> GSHMGNRTFSYTLED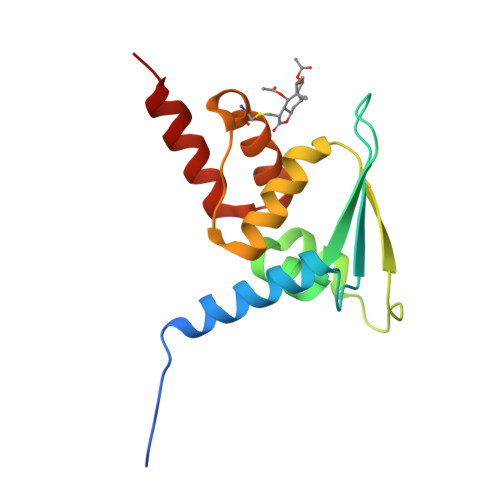HTKQAFGIMNELRLSQQLCDVTLQVKYQDAPAAQFMAHKVVLASSSPVFKAMFTNGLREQGMEVVSIEGIHPKVMERLIEFAYTASISMGEKCVLHVMNGAVMYQIDSVVRACADFLVQQLD> TCCG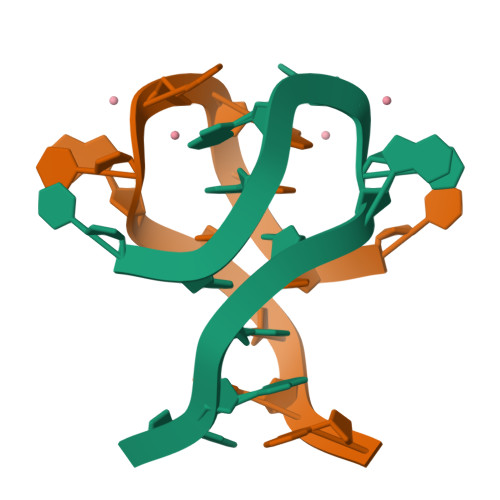CCGCCGA> GSHMAHAGRTGYDNREIVMKYIHYKLSQRGYEWDAGDDVEENRTEAPEGTESEVVHLTLRQAGDDFSRRYRRDFAEMSSQLHLTPFTARGRFATVVEELFRDGVNWGRIVAFFEFGGVMCVESVNREMSPLVDNIALWMTEYLNRHLHTWIQDNGGWD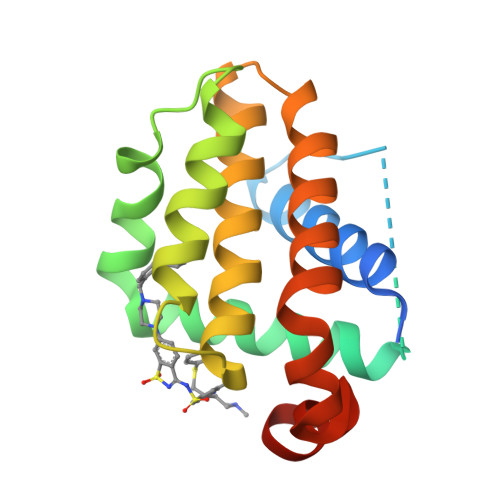AFVELYGPSMR>MKTINSVDTKEFLNHQVANLNVFTVKIHQIGWYMRGHNFFTLHEKMDDLYSEFGEQMDEVAERLLAIGGSPFSTLKEFLENASVEEAPYTKPKTMDQLMEDLVGTLELLRDEYK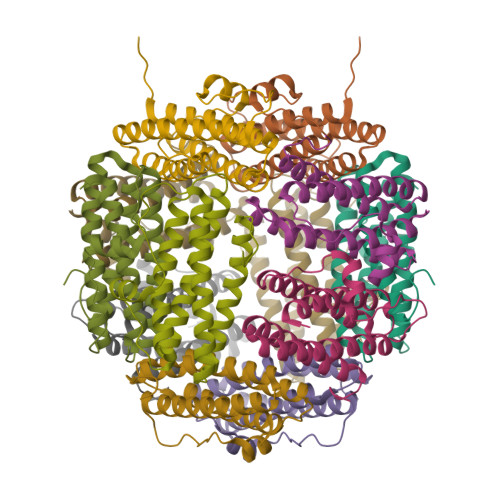QGIELTDKEGDDVTNDMLIAFKASIDKHIWMFKAFLGKAPLE[6x]>MKKLVLLMLVLLLVYPHVSKAGGFKGGGGNPGYWFAGDPVEHPDPAKPPIVFVHGLNGSSSAWFDENDMAEQAWKNGYDAAFIDLHPDKDMQDNGAMLAAKLREIYQYFGRKVILVSYSKGGIDSQSALIHHNAYHYVERVITLGTPHHGSQLADLAYSNWAGWLADILGQKNDAVYSLQTGFMKSFRDQTDNHPNRLKTKYFTLAGNKIGGFGSALFFGGVYLNMFGENDGAVTEKNARLPYATNLDTGKWDHFSIIKGNLTFPVFMPLLTIQANANETAATKENLSYPFIRGGENHGLREEEFAVEKGVKEITVHWLSNHSSGNIKLTDPRGKPFKDFSIAKTADVFEGGFVHSA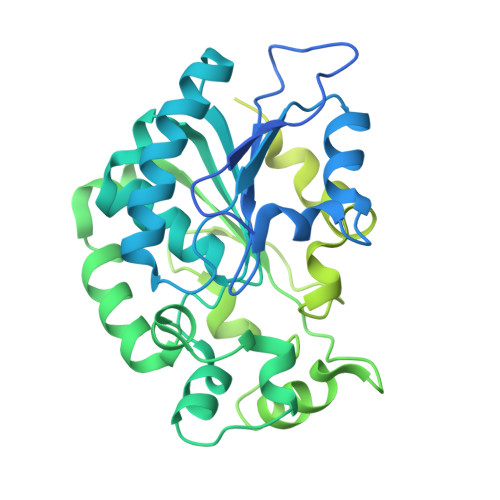AIKNPAAGTWKIASSVKQKEAFLFIVTFDSPLNQQIKNAVTRESSNLANVKASVRSIRYENGKQAEKKSLKPASINALQNSLSFKKAGMYSVTIDLSGKTADNSPFNRTIIRSIYVNDKGEKFENSPLSD[6x]N,N-dimethylquinoxaline-6-carboxamide | C11 H11 N3 O | 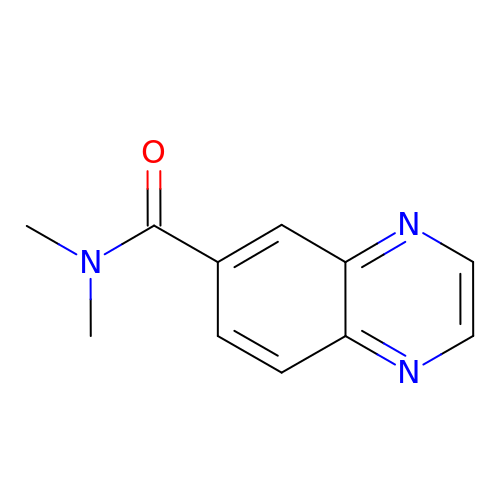HQOVESVNZPVFDO-UHFFFAOYSA-N Expression of the putative acr on a plasmid in a CR1-immunized S. thermophilus strain completely abolished immunity against the CRISPR-sensitive virulent phage D5842 (green), and even eliminated the residual resistance observed against phage D1811 (red). This new Acr, which bears no similarity to any Acr characterized to date, was named AcrIIA6. All AcrIIA6 and AcrIIA5 orthologs completely restored the plaquing efficiency of phages targeted by the CR1 system of S. thermophilus, indicating they are blocking the activity of St1Cas9. AcrIIA6s did not impede SpCas9, while AcrIIA2 and AcrIIA4 exhibited only a partial inhibition.

With bioinformatic predictions yielding little information, we set about the biochemical characterization of AcrIIA6. It crystallized readily and its structure was solved at 1.96 Å revealing a dimeric assembly. Gel filtration profiles also indicated that AcrIIA6 is a dimer in solution. Each monomer consists of eight α-helices and four β-strands forming a β-sheet, with the sequence topology α1α2α3α4α5α6α7β1β2β3β4α8. When the AcrIIA6 structure was submitted to the DALI server, only low scores of structural similarity were returned. The superimposition of the AcrIIA6 HTH dimer onto the C.Esp1396I-dsDNA complex brings the AcrIIA6 helix 3 into contact with the two major grooves of the dsDNA. Helix 3 exhibits strong electropositivity, a feature observed in dsDNA binding helices, including the one from C.Esp1396I. We mapped the sequence conservation among the 48 unique AcrIIA6 alleles to the structure obtained. The dimerization interface is largely conserved as are the DNA-interacting arms of the HTH motif. For AcrIIA6, we chose an ortholog (92% ID) from the reference phage DT139 whose host, SMQ-301, also contains both CR1 and CR3 systems.

>[2x]MKINDDIKELILEYMSRYFKFENDFYKLPGIKFTDANWQKFKNGGTDIEKMGAARVNAMLDCLFDDFELAMIGKAQTNYYNDNSLKMNMPFYTYYDMFKKQQLLKWLKNNRDDVIGGTGRMYTASGNYIANAYLEVALESSSLGSGSYMLQMRFKDYSKGQEPIPSGRQNRLEWIENNLENIRLE>[3x]MDFSRFFIDRPIFAAVLSILIFITGLIAIPLLPVSEYPDVVPPSVQVRAEYPGANPKVIAETVATPLEEAING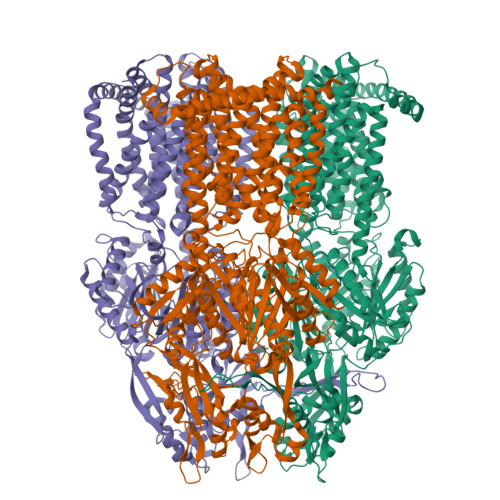VENMMYMKSVAGSDGVLVTTVTFRPGTDPDQAQVQVQNRVAQAEARLPEDVRRLGITTQKQSPTLTLVVHLFSPNGKYDSLYMRNYATLKVKDELARLPGVGQIQIFGSGEYAMRVWLDPNKVAARGLTASDVVTAMQEQNVQVSAGQLGAEPLPQESDFLISINAQGRLHTEEEFGNIILKTAQDGSLVRLRDVARIEMGSGSYALRSQLNNKDAVGIGIFQSPGANAIDLSNAVRAKMAELATRFPEDMQWAAPYDPTVFVRDSIRAVVQTLLEAVVLVVLVVILFLQTWRASIIPLIAVPVSVVGTFSILYLLGFSLNTLSLFGLVLAIGIVVDDAIVVVENVERNIEEGLAPLAAAHQAMREVSGPIIAIALVLCAVFVPMAFLSGVTGQFYKQFAVTIAISTVISAINSLTLSPALAALLLKPHGAKKDLPTRLIDRLFGWIFRPFNRFFLRSSNGYQGLVSKTLGRRGAVFAVYLLLLCAAGVMFKVVPGGFIPTQDKLYLIGGVKMPEGSSLARTDAVIRKMSEIGMNTEGVDYAVAFPGLNALQFTNTPNTGTVFFGLKPFDQRKHTAAEINAEINAKIAQIQQGFGFSILPPPILGLGQGSGYSLYIQDRGGLGYGALQSAVNAMSGAIMQTPGMHFPISTYQANVPQLDVQVDRDKAKAQGVSLTELFGTLQTYLGSSYVNDFNQFGRTWRVMAQADGPYRESVEDIANLRTRNNQGEMVPIGSMVNISTTYGPDPVIRYNGYPAADLIGDADPRVLSSSQAMTHLEELSKQILPNGMNIEWTDLSFQQATQGNTALIVFPVAVLLAFLVLAALYESWTLPLAVILIVPMTMLSALFGVWLTGGDNNVFVQVGLVVLMGLACKNAILIVEFARELEIQGKGIMEAALEACRLRLRPIVMTSIAFIAGTIPLILGHGAGAEVRGVTGITVFSGMLGVTLFGLFLTPVFYVTLRKLVTRRKPVQEDLPAHHHHHH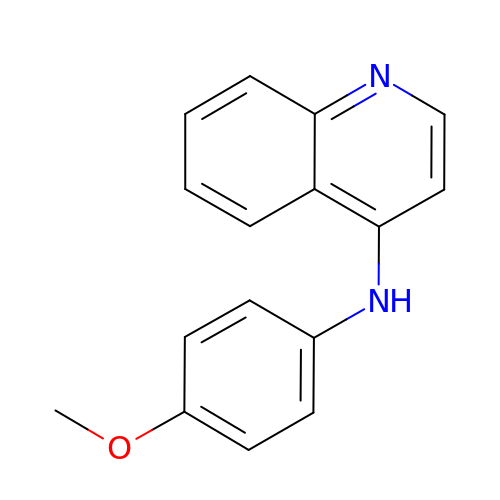N-(4-methoxyphenyl)quinolin-4-amine | C16 H14 N2 O | XEXJCSNBUIARJF-UHFFFAOYSA-N methylthioacryloyl-CoA | 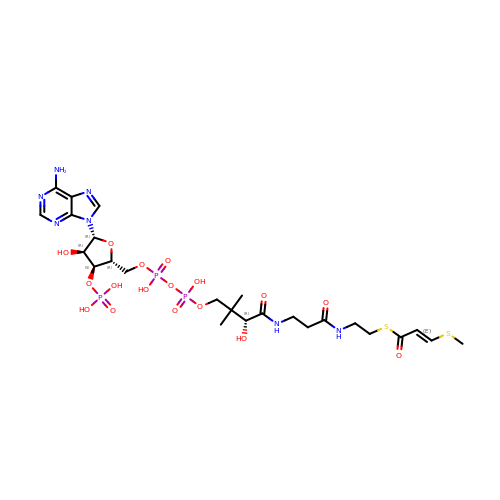C25 H40 N7 O17 P3 S2 | ZGBNNHAIMKRDOC-CABWFRLRSA-N>[2x]MNIQKSENKANPQKLVVALLPDESAATVIQNNKGLEMYLENKLNKDIELFVSTDYSSMIEVASKGRLDLAYFGPLSYVLAKTKSNIEPFAALEKDGKNTYQALVIGNAEAGINSYEKIEGKIMAYGDQASTSSHLIPKSMLKQKQLKAGENYEEVFVGAHDAVAIAVANGKAQAGGLSKPIFTALIERGTIDKNKVII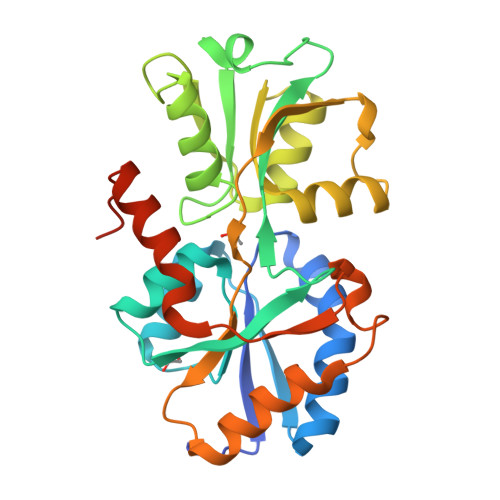IAESKPFPQYPWTMRSDLDSELKTQIQQAFLELEDKAILKPFKADAFTLVTDQDYDVVRNLGEVLELNFEQLNKLEHHHHHH>[3x]MKFSKEQFDYSLYLVTDSGMIPEGKTLYGQVEAGLQNGVTLVQIREKDADTKFFIEEALQIKELCHAHNVPLIINDRIDVAMAIGADGIHVGQDDMPIPMIRKLVGPDMVIGWSVGFPEEVDELSKMGPDMVDYIGVGTLFPTLTKKNPKKAPMGTAGAIRVLDALERNNAHWCRTVGIGGLHPDNIERVLYQCVSSNGKRSLDGICVVSDIIASLDAAKSTKILRGLIDKTDYKFVNIGLSTKNSLTTTDEIQSIISNTLKARPLVQHITNKVHQNFGANVTLALGSSPIMSEIQSEVNDLAAI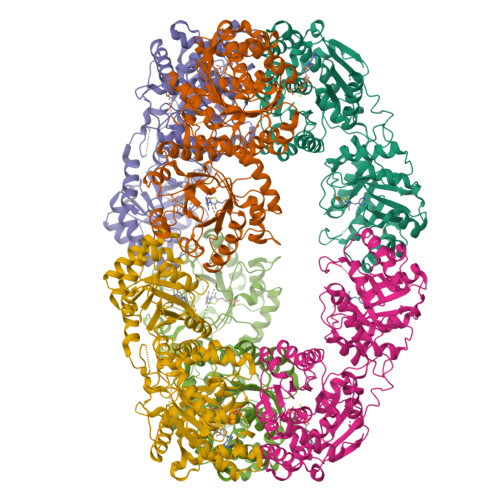PHATLLLNTGSVAPPEMLKAAIRAYNDVKRPIVFDPVGYSATETRLLLNNKLLTFGQFSCIKGNSSEILGLAELNKERMKGVDASSGISNELLIQATKIVAFKYKTVAVCTGEFDFIADGTIEGKYSLSKGTNGTSVEDIPCVAVEAGPIEIMGDITASGCSLGSTIACMIGGQPSEGNLFHAVVAGVMLYKAAGKIASEKCNGSGSFQVELIDALYRLTRENTPVTWAPKLTHT>MLEQPIGVIDSGVGGLTVAKEIMRQLPKENIIYVGDTKRCPYGPRPEEEVLQYTWELTNYLLENHHIKMLVIACNTATAIALDDIQRSVGIPVVGVIQPGARAAIKVTDNQHIGVIGTENTIKSNAYEEALLALNPDLKVENLACPLLVPFVESGKFLDQTADEIVKTSLYPLKDTSIDSLILGCTHYPILKEAIQRYMGEHVNIISSGDETAREVSTIL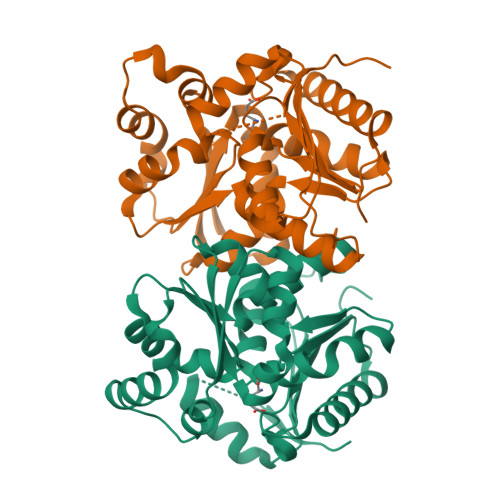SYKGLLNQSPIAPDHQFLTTGARDQFAKIADDWFGHEVGHVECISLQEPIKR[3x]> GSTGSTDSPTQPTTGSFCPGPVTLCSDLESHSTEAVLGDALVDFSLKLYHAFSAMKKVETNMAFSPFSIASLLTQVLLGAGENTKTNLESILSYPKDFTCVHQALKGFTTKGVTSVSQIFHSPDLAIRDTF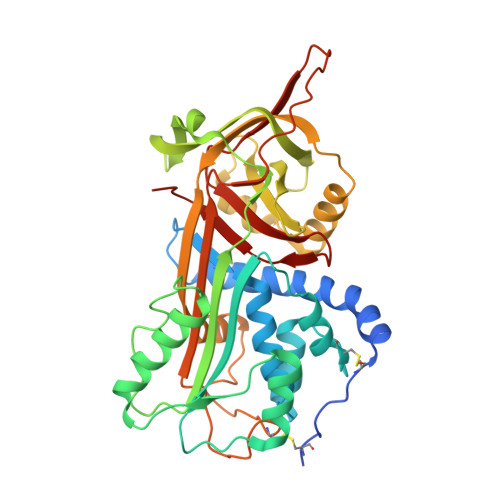VNASRTLYSSSPRVLSNNSDANLELINTWVAKNTNNKISRLLDSLPSDTRLVLLNAIYLSAKWKTTFDPKKTRMEPFHFKNSVIKVPMMNSKKYPVAHFIDQTLKAKVGQLQLSHNLSLVILVPQNLKHRLEDMEQALSPSVFKAIMEKLEMSKFQPTLLTLPRIKVTTSQDMLSIMEKLEFFDFSYDLNLCGLTEDPDLQVSAMQHQTVLELTETGVEAAAASAISVARTLLVFEVQQPFLFVLWDQQHKFPVFMGRVYDPRA> XMQKYV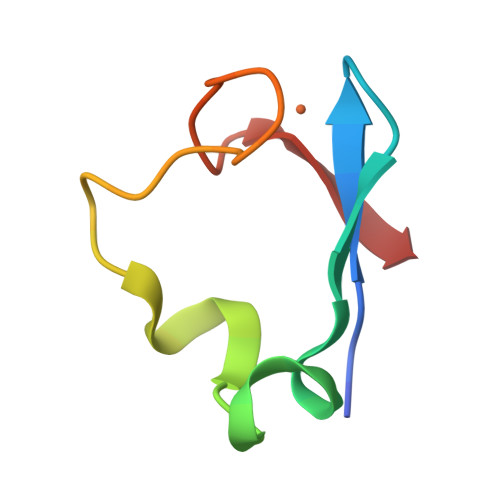CNVCGYEYDPAEHDNVPFDQLPDDWCCPVCGVSKDQFSPA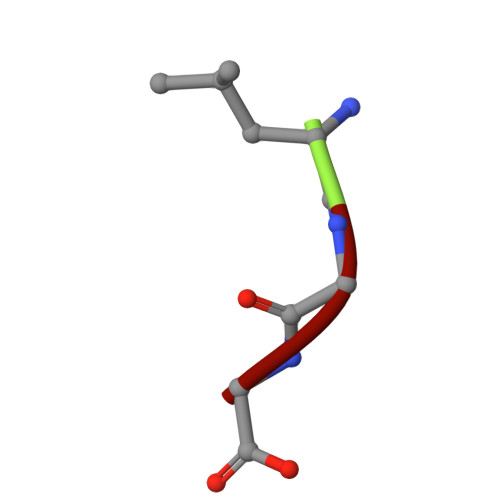> LGG> SCA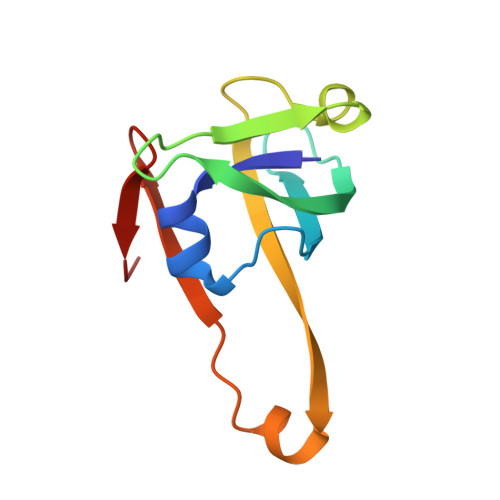IDQDFLDAAGILENEAIDIWNVTNGKRFSTYAIAAERGSRIISVNGAAAHCASVGDIVIIASFVTMPDEEARTWRPNVAYFEGDNEMKRTA>[2x]TGMSREEVESLIQEVLEVYPEKARKDRNKHLAVNDPAVTQSKKCIISNKKSQPGLMTIRGCAYAGSKGIVWGPIKDMIHISHGPVGCGQYSRAGRRNYYIGTTGVNAFVTMNFTSDFQEKDIVFGGDKKLAKLIDEVETLFPLNKGISVQSECPIGLIGDDIESVSKVKGAELSKTIVPVRCEGFRGVSQSLGHHIANDAVRDWVLGKRDEDTTFASTPYDVAIIGDYNIGGDAWSSRILLEEMG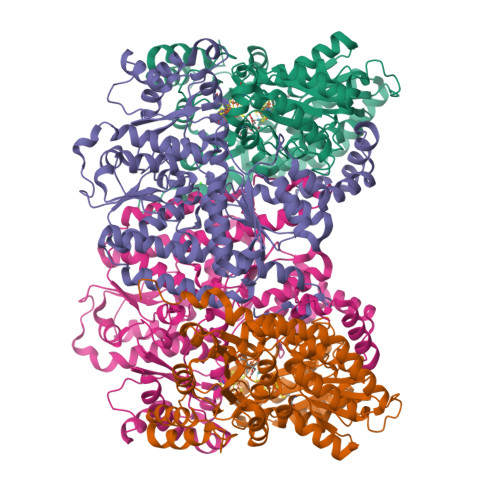LRCVAQWSGDGSISEIELTPKVKLNLVHCYRSMNYISRHMEEKYGIPWMEYNFFGPTKTIESLRAIAAKFDESIQKKCEEVIAKYKPEWEAVVAKYRPRLEGKRVMLYIGGLRPRHVIGAYEDLGMEVVGTGYEFAHNDDYDRTMKEMGDSTLLYDDVTGYEFEEFVKRIKPDLIGSGIKEKFIFQKMGIPFREMHSWDYSGPYHGFDGFAIFARDMDMTLNNPCWKKLQAPWEASEGAEKVAASA;>[2x]SQQVDKIKASYPLFLDQDYKDMLAKKRDGFEEKYPQDKIDEVFQWTTTKEYQELNFQREALTVNPAKACQPLGAVLCALGFEKTMPYVHGSQGCVAYFRSYFNRHFREPVSCVSDSMTEDAAVFGGQQNMKDGLQNCKATYKPDMIAVSTTCMAEVIGDDLNAFINNSKKEGFIPDEFPVPFAHTPSFVGSHVTGWDNMFEGIARYFTLKSMDDKVVGSNKKINIVPGFETYLGNFRVIKRMLSEMGVGYSLLSDPEEVLDTPADGQFRMYAGGTTQEEMKDAPNALNTVLLQPWHLEKTKKFVEGTWKHEVPKLNIPMGLDWTDEFLMKVSEISGQPIPASLTKERGRLVDMMTDSHTWLHGKRFALWGDPDFVMGLVKFLLELGCEPVHILCHNGNKRWKKAVDAILAASPYGKNATVYIGKDLWHLRSLVFTDKPDFMIGNSYGKFIQRDTLHKGKEFEVPLIRIGFPIFDRHHLHRSTTLGYEGAMQILTTLVNSILERLDEETRGMQATDYNHDLVR> MAHHHHHHMLRIGLTGGIGAGKSALSSAFAQCGAVIVDGDVIAREVVRPGTEGLAALVEAFGRDILLADGSLDRPALAAKAFADDAARQTLNGIVHPLVGARRAEIIASVPADSVVVEDIPLLVESGMAPLFPLVVIVYADVEVRLRRLVEQRGMAEADARARIAAQASDEQRRAVADIWLDNSGSPAELVQRAQQVWNERIVPFAHNLSTRQIARAPVRLVPPDPEWPAQAQRIVNRLKTASGHRALRVDHVGSTALPGDPDFAAKDVIDIQITVESLAAADELVEPLLAAGYPRLEHITADVAKPDARSTVERYDHTGDPALWHKRIHASADPGRPTNVHIRVDGWPGQQFALLFVDWLTADP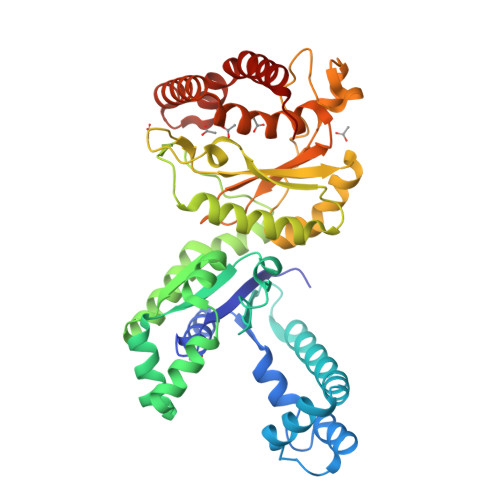DARADYLAVKRSAEQRADGDIDAYVAVKEPWFRDAYRRAWDWADSTGWKP>[2x]MAASLPSTLSFSSAPDEIQHPQIKFSEWKFKLFRVRSFEKAPEEAQKEKDSSEGKPYLEQSPVVPEKPGGQNSILTQRALKLHPKFSKKFHADGKSSDKAVHQARLRHFCRICGNRFKSDGHSRRYPVHGPVDAKTQSLFRKKEKRVTSWPDLIARIFRIDVKADVDSIHPTEFCHDCWSIMHRKFSSSHSQVYFPRKVTVEWHPHTPSCDICFTAHRGLKRKRHQPNVQLSKKLKTVLNHARRDRRKRTQARVSSKEVLKKISNCSKIHLSTKLLAVDFPAHFVKSISCQICEHILADPVETSCKHLFCRICILRCLKVMGSYCPSCRYPCFPTDLESPVKSFLNILNSLMVKCPAQDCNEEVSLEKYNHHVSSHKESKETLVHINKGGRPRQHLLSLTRRAQKHRLRELKIQVKEFADKEEGGDVKAVCLTLFLLALRARNEHRQADELEAIMQGRGSGLQPAVCLAIRVNTFLSCSQYHKMYRTVKAITGRQIFQPLHALRNAEKVLLPGYHPFEWQPPLKNVSSRTDVGIIDGLSGLASSVDEYPVDTIAKRFRYDSALVSALMDMEEDILEGMRSQDLDDYLNGPFTVVVKESCDGMGDVSEKHGSGPAVPEKAVRFSFTVMRITIEHGSQNVKVFEEPKPNSELCCKPLCLMLADESDHETLTAILSPLIAEREAMKSSELTLEMGGIPRTFKFIFRGTGYDEKLVREVEGLEASGSVYICTLCDTTRLEASQNLVFHSITRSHAENLQRYEVWRSNPYHESVEELRDRVKGVSAKPFIETVPSIDALHCDIGNAAEFYKIFQLEIGEVYKHPNASKEERKRWQATLDKHLRKRMNLKPIMRMNGNFARKLMTQETVDAVCELIPSEERHEALRELMDLYLKMKPVWRSSCPAKECPESLCQYSFNSQRF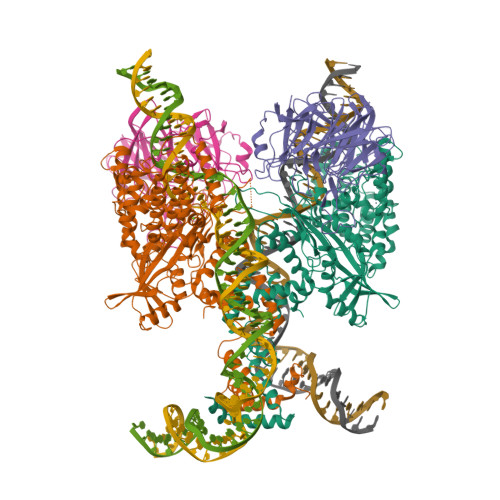AELLSTKFKYRYEGKITNYFHKTLAHVPEIIERDGSIGAWASEGNQSGNKLFRRFRKMNARQSKCYEMEDVLKHHWLYTSKYLQKFMNAHNALKSSGFTMNSKETLGDPLGIEDSLESQDSMEF;>[2x]MSLQMVTVGHNIALIQPGFSLMNFDGQVFFFGQKGWPKRSCPTGVFHFDIKQNHLKLKPAIFSKDSCYLPPLRYPATCSYKGSIDSDKHQYIIHGGKTPNNELSDKIYIMSVACKNNKKVTFRCTEKDLVGDVPEPRYGHSIDVVYSRGKSMGVLFGGRSYMPSTQRTTEKWNSVADCLPHVFLIDFEFGCATSYILPELQDGLSFHVSIARNDTVYILGGHSLASNIRPANLYRIRVDLPLGTPAVNCTVLPGGISVSSAILTQTNNDEFVIVGGYQLENQKRMVCSLVSLGDNTIEISEMETPDWTSDIKHSKIWFGSNMGNGTIFLGIPGDNKQAMSEAFYFYTLRCSEEDLSEDQKIVSNSQTSTEDPGDSTPFEDSEEFCFSAEATSFDGDDEFDTYNEDDEDDESVTGYWITCCPTCDVDINTWVPFYSTELNKPAMIYCSHGDGHWVHAQCMDLEERTLIHLSEGSNKYYCNEHVQIARALQTPKRNPPLQKPPMKSLHKKGSGKVLTPAKKSFLRRLFD> MHHHHHHMGSVQRQDLVLFSDQS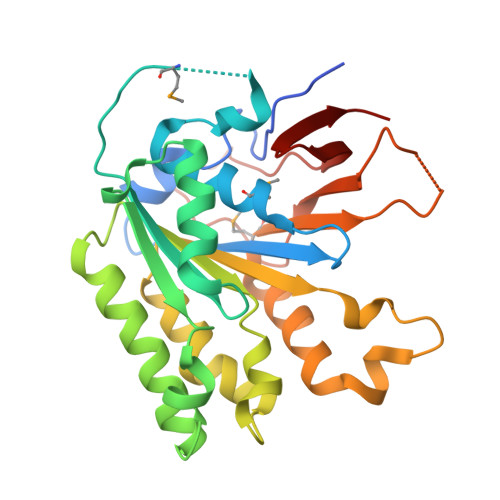VLPAHFFQDSNSHNLFFITHQSCTQPLWMINALVETHVLGSPSSLNESSSSMLPSSTRSHAVLASFIHEQNYFTNSLNKLKIPSNNYNVLDFLSDFIVNNIHNKPRDKILSDVLAKFSAAIQNNPTDTIVIIEQPELLLSLVSGLTCSELNNKFITPLLRQCKVLIIVSNSDIFNIDEYDASVHSSNLQNFYKSSFIKSMINLNLNPLKTGFAKDVTGSLHVCRGGAPIATSNTSLHVVENEYLYLNEKESTKLFYR>PGSSGLPPEKPKNLSCIVNEGKKMRCEWDGGRETHLETNFTLKSEWATHKFADCKAKRDTPTSCTVDYSTVYFVNIEVWVEAENALGKVTSDHINFDPVYKVKPNPPHNLSVINSEELSSILKLTWTNPSIKSVIILKYNIQYRTKDASTWSQIPPEDTASTRSSFTVQDLKPFTE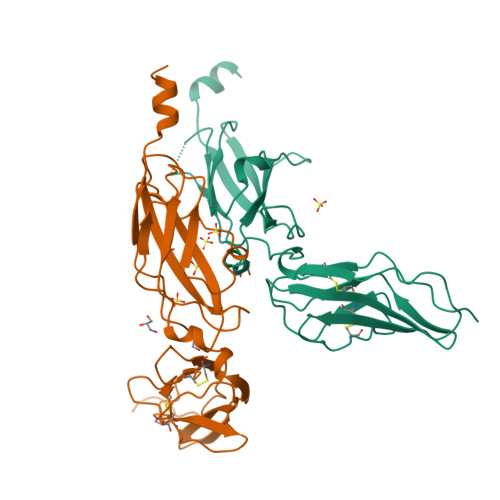YVFRIRCMKEDGKGYWSDWSEEASGITYEDRPSKEPSFW[2x]> SRANDAPIVLLHGFTGWGREEMFGFKYWGGVRGDIEQWLNDNGYRTYTLAVGPLSSNWDRACEAYAQLVGGTVDYGAAHAAKHGHARFGRTYPGLL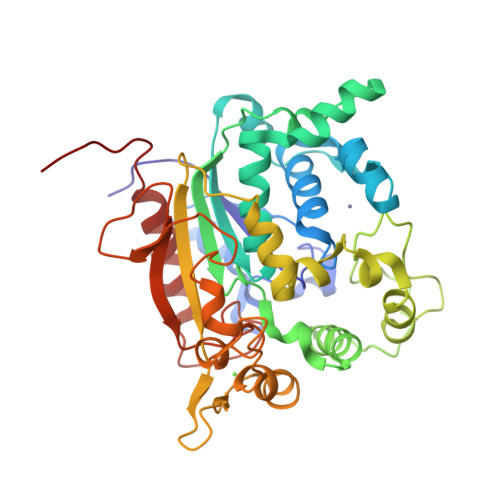PELKRGGRIHIIAHSQGGQTARMLVSLLENGSQEEREYAKAHNVSLSPLFEGGHHFVLSVTTIATPHDGTTLVNMVDFTDRFFDLQKAVLKAAAVASNVPYTSQVYDFKLDQWGLRRQPGESFDQYFERLKRSPVWTSTDTARYDLSVPGAEKLNQWVKASPNTYYLSFATERTYRGALTGNYYPELGMNAFSAVVCAPFLGSYRNATLGIDDRWLENDGIVNAFSMNGPKRGSTDRIVPYDGTIKKGVWNDMGTYNVDHFEVIGVDPNPLFDIRAFYLRLAEQLASLQPHHHHHH>[4x]SMTNLQTFELPTEVTGCAADISLGRALIQAWQKDGIFQIKTDSEQDRKTQEAMAASKQFCKEPLTFKSSCVSDLTYSGYVASGEEVTAGKPDFPEIFTVCKDLSVGDQRVKAGWPCHGPVPWPNNTYQKSMKTFMEELGLAGERLLKLTALGFELPINTFTDLTRDGWHHMRVLRFPPQTS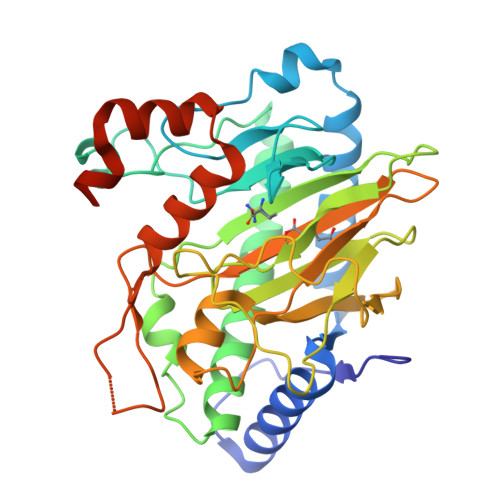TLSRGIGAHTEYGLLVIAAQDDVGGLYIRPPVEGEKRNRNWLPGESSAGMFEHDEPWTFVTPTPGVWTVFPGDILQFMTGGQLLSTPHKVKLNTRERFACAYFHEPNFEASAYPLFEPSANERIHYGEHFTNMFMRCYPDRITTQRINKENRLAHLEDLKKYSDTRATGS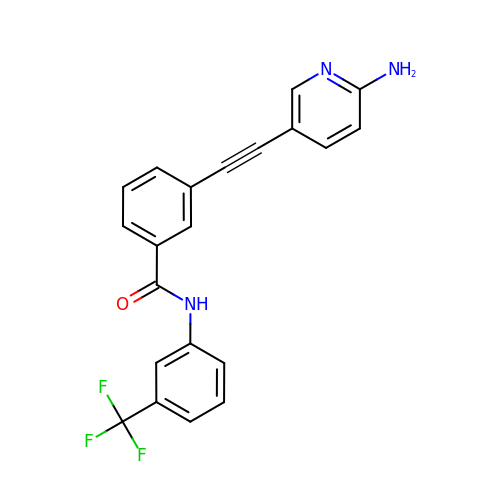3-[(6-aminopyridin-3-yl)ethynyl]-N-[3-(trifluoromethyl)phenyl]benzamide | C21 H14 F3 N3 O | MWTXIEKNSGTHCF-UHFFFAOYSA-N> EATAGTVTVNAITSDDTIDGIELGQTISISGKAVGGDISVGDVVKMTINNTEYSTTVKAGGIWMIAGVLGSDLAADSEFDVVVTSSDAAGNKVQSIGTSTHSVDLSAEANFSLAEGQQHVLTNLPEGFGFPDGTTEVVTNFGGTITLGDDGEYRYDAPVRDHGDAVSDKDSVTVTLEDGRTFTVNLDIQDSAPVAVDDQDSIVVQHEEFEVSEIAASWVSYTHGESVTTFDGTSDLGGVDNDSAKDQIRWGNPAESKQSGYGFIDNDSNLEGRFDLNQDISVGTFTHYNYPVYSGGAITSAEMSVEFSVLDHLGVSTPVTLTVNFDHNETPNTNDVNASRDIVTVQNTHVTFERDGDIYTVQIVGFREVGNPDGEVVTSIYTNENAATSYELVVRVVEGDGYSLPSTEGNIFDDNGLGADSLGADGSVTVVGVAVGAIVSSNESVGHSIEGQYGNLVLNSDG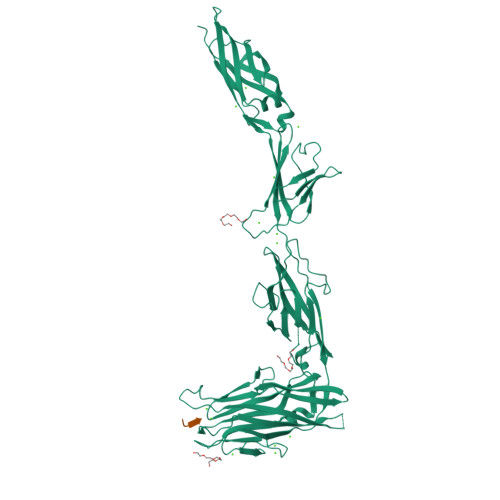SYVYDVTASVSDIPAGATESFAYLIQDQDGSTSSANLSINVGTN;> GYTS>MEIPVIEPLF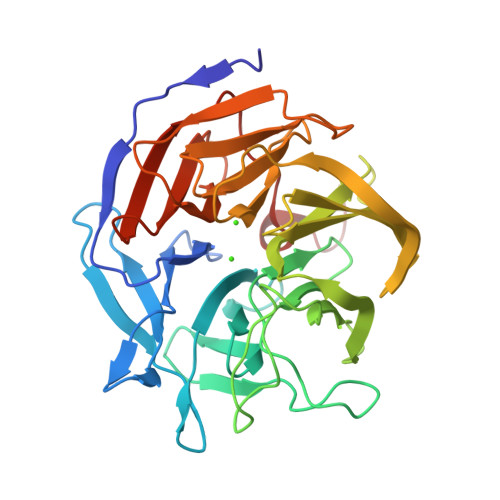TKVTEDIPGAEGPVFDKNGDFYIVAPDVEVNGKPAGEILRIDLKTGKKTVICKPEVNGYGGIPAGCQCDRDANQLFVADMRLGLLVVQTDGTFEEIAKKDSEGRRMQGCNDCAFDYEGNLWITAPAGEVAPADATASMQEKFGSIYCFTTDGQMIQVDTAFQFPNGIAVRHMNDGRPYQLIVAEMPTKKLWSYDIKGPAKIENKKVWGHIPGTHEGGADGMDFDEDNNLLVANWGSSHIEVFGPDGGQPKMRIRCPFEKPSNLHFKPQTKTIFVTEHENNAVWKFEWQRNGKKQYCETLKFGIF[4x]>MAHHHHHHTSTLMGSLTMLGKAGCQWEHANTSFASFSNVVACNTATVTGLASAPTEGKIPGIRFANLPAGDYELTVLIFSMYPVDAGVYCRYRLWDGTNFSGMAGAYESEIYQMTGLFSYATDQTNLTFYVQAQTLTATKNCRADITVPGQDKMQIYLKKL[3x]

Bdellovibrio bacteriovorus is a bacterium that preys upon a wide range of other Gram-negative bacteria, entering their periplasm and consuming them from within. Proteomic and structural analyses of vesicle contents reveal several fibre-like proteins, which we name the mosaic adhesive trimer (MAT) superfamily, and show localization on the predator surface before prey encounter. Structural studies reveal a variety of domain usages (and therefore binding capabilities) at the fibre C-termini, placing these on intertwined trimeric β-prisms. Using independent but complementary approaches, we identified and characterized a MAT superfamily of trimeric fibre proteins with diverse adhesive tips, able to fulfil the long-sought-after role of multiplicity of molecular recognition and handling of diverse epitopes (across a wide prey range), by the bacterial predator B. bacteriovorus.

We next characterized two more divergent NS74s, Bd2439 and Bd2734, obtaining a tip-only variant of Bd2734 (residues T691–L843, 1.8 Å) and a longer construct of Bd2439 (G837–D1107, 1.6 Å). The resulting structures reveal that both proteins use a related fold. The Bd2734 tip represents a divergent TNF fold, with large pockets between monomers. Superimposing with a Burkholderia lectin–fucose complex25 shows how the Bd2734 pocket can accommodate a terminal monosaccharide. We found that Bd2740–mCherry did locate to the CpoBBd0635-containing vesicle, deposited during predatory invasion, while Bd1334–mCherry and Bd2734–mCherry fluorescence were diffuse throughout the B. bacteriovorus cell. However, a slight reduction in prey entry efficiency was seen for deletion mutants of Bd2734 and Bd2740, which are structurally divergent but have similar expression profiles and are encoded at nearby genetic loci. Bd2734 and Bd2740 are two of the shorter MAT fibres (843 and 627 aa, respectively), which are relevant given that one of the short MATs we were unable to crystallize (Bd2872, 626 aa) was previously identified in a screen for predation-deficient mutants.> MAREVKLTKAGYERLMQQLERER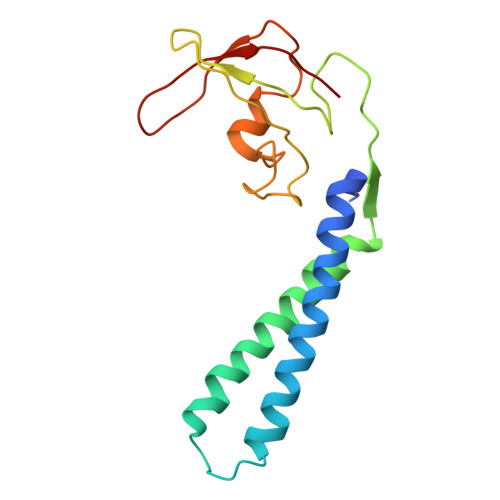ERLQEISADFEQALEEGDLRENAGYDEARRAMWQNEARIDSLEDILSRAVILEEGSGEVIGLGSVVELEDPLSGERLSVQVVSPAEANVLDTPMKISDASPMGKALLGHRVGDVLSLDTPKGRREFRVVAIHG> QGPLGSSEQLKHCNGILKELLSKKHAAYAWPFYKPVDASALGLHDYHDIIKHPMDLSTVKRKMENRDYRDAQEFAADVRLMFSNCYKYNPPDHDVVAMARKLQDVFEFRYAKMPD;> XWWIIPKVKKGCX

Within this class of proteins, the bromodomain and extraterminal domain (BET) family contains four members that are transcriptional coregulators and that recognize acetyllysines (AcKs) using a tandem pair of highly homologous bromodomains (BDs). Despite heavy academic and industry investment in this area, the generation of paralog-selective inhibitors has proved elusive because of the extremely high sequence similarity between the bromodomains of family members (90 to 95% within the acetyllysine-binding pocket residues). Using the highly conserved BET BDs as a model system, we conducted three mRNA display-based RaPID (random nonstandard peptides integrated discovery) screens using a single library (which contains >1012 unique members). Crystal structures of 13 distinct peptide–bromodomain complexes revealed highly diverse structures and binding modes among the cyclic peptide ligands.

Overall, the peptide backbone itself adopts the same conformation and all intermolecular contacts in the AcK-binding region are also conserved. Minor differences are a 180° flip of the Trp1 side chain and a change in the nature of the contacts made between AcK9 and the C-terminal part of helix αZ and N-terminal part of helix αD in the BD, which is distal to the main AcK pocket (a region less conserved between BD1 and BD2 domains). In the structures with BD1 domains, this AcK lies within a channel formed between conserved Phe (in the loop following αZ) and Asp (αD) residues. A tyrosine residue replaces the Phe in BD2 domains and is positioned in the opposite direction to the Asp, leading to a loss of this groove. As a result, AcK9 is oriented toward the solvent in our structure of the peptide with BRD2-BD2. This difference likely contributes to the significant differences in affinity for the two domains, illustrating the power of such peptides to achieve specificity by probing surfaces beyond the canonical binding pocket.> QVKDFVIEPPIKNNLHIYKTFGVFGGKEYSANSMYLVTKKGVVLFDVPWEKVQYQSLMDTIKKRHNLPVVAVFATHSHDDRAGDLSFFNNKGIKTYATAKTNEFLKKDGKATSTEIIKTGKPYRIGG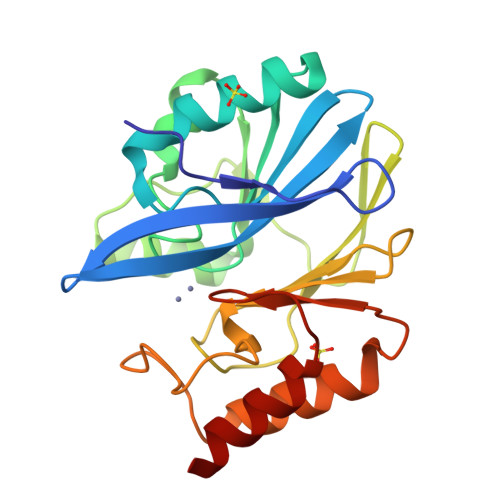EEFVVDFLGEGHTADNVVVWFPKYNVLDGGCLVKSNSATDLGYIKEANVEQWPKTINKLKAKYSKATLIIPGHDEWKGGGHVEHTLELLNKK1-cyclopropyl-~{N}-[2-[[(2~{S})-2-methylpyrrolidin-1-yl]methyl]-3~{H}-benzimidazol-5-yl]indazole-5-carboxamide | C24 H26 N6 O 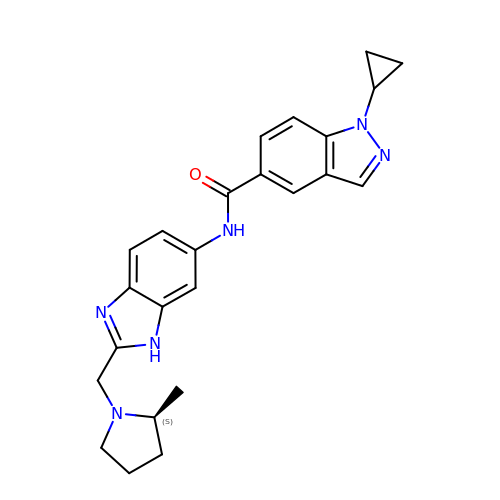| FTNYJPRHIRILOI-HNNXBMFYSA-N>[4x]AKKEIPLKYGATNEGKRQDPAMQKFRDNRLGAFIHWGLYAIPGGEWNGKVYGGAAEWLKSWAKVPADEWLKLMDQWNPTKFDAKKWAKMAKEMGTKYVKITTKHHEGFCLWPSKYTKYTVANTPYKRDILGELVKAYNDEGIDVHFYFSVMDWSNPDYRYDIKSKEDSIAFSRFLEFTDNQLKELATRYPTVKDF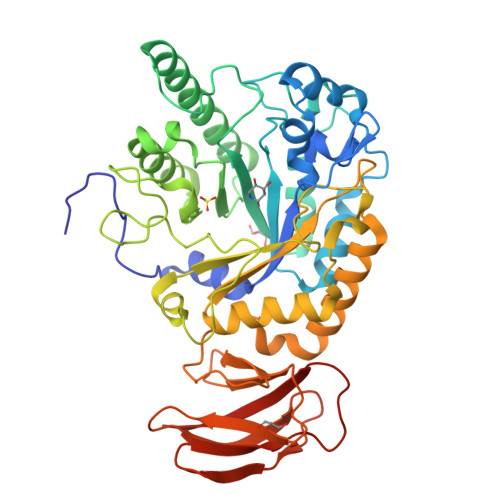WFDGTWDASVKKNGWWTAHAEQMLKELVPGVAINSRLRADDKGKRHFDSNGRLMGDYESGYERRLPDPVKDLKVTQWDWEACMTIPENQWGYHKDWSLSYVKTPIEVIDRIVHAVSMGGNMVVNFGPQADGDFRPEEKAMATAIGKWMNRYGKAVYACDYAGFEKQDWGYYTRGKNDEVYMVVFNQPYSERLIVKTPKGITVEKATLLTTGEDITVVETTRNEYNVSVPKKNPGEPYVIQLKVRAAKGTKSIYRDALT7,8-DIHYDROXY-1-METHOXY-3-METHYL-10-OXO-4,10-DIHYDRO-1H,3H-PYRANO[4,3-B]CHROMENE-9-CARBOXYLIC 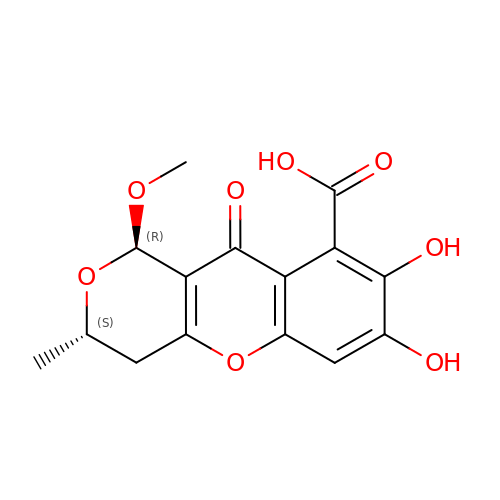ACID | C15 H14 O8 | RSFJMLCZHPZXCW-AANKLQPISA-N> MKRKTKIVSTIGPASESVDKLVQLMEAGMNVARLNFSHGDHEEHGRRIANIREAAKRTGRTVAILLDTKGPEIRTHNMENGAIELKEGSKLVISMSEVLGTPEKISVTYPSLIDDVSVGAKILLDDGLISLEVNAVDKQAGEIVTTVLNGGVLKNKKGVNVPGVKVNLPGITEKDRADILFGIRQGIDFIAASFVRRASDVLEIRELLEAHDALHIQIIAKIENE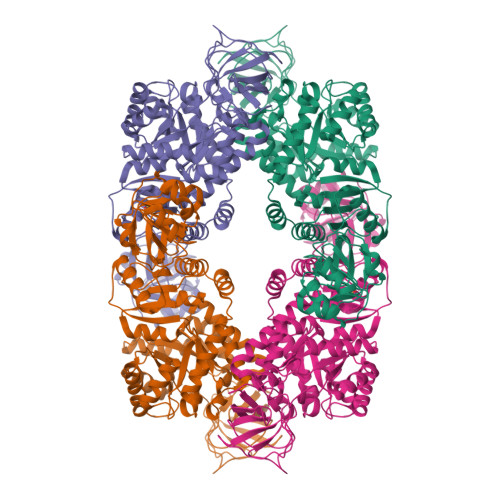EGVANIDEILEAADGLMVARGDLGVEIPAEEVPLIQKLLIKKSNMLGKPVITATQMLDSMQRNPRPTRAEASDVANAIFDGTDAVMLSGETAAGQYPVEAVKTMHQIALRTEQALEHRDILSQRTKESQTTITDAIGQSVAHTALNLDVAAIVTPTVSGKTPQMVAKYRPKAPIIAVTSNEAVSRRLALVWGVYTKEAPHVNTTDEMLDVAVDAAVRSGLVKHGDLVVITAGVPVGETGSTNLMKVHVISDLLAKGQGIGRKSAFGKAVVAKTAEEARQKMVDGGILVTVSTDADMMPAIEKAAAIITEEGGLTSHAAVVGLSLGIPVIVGVENATTLFKDGQEITVDGGFGAVYRGHASVL>[4x]SMRNVALITGITGQDGSYLAEFLLEKGYEVHGIVRRSSSFNTGRIEHLYKNPQAHIEGNMKLHYGDLTDSTCLVKIINEVKPTEIYNLGAQSHVKISFDLAEYTADVDGVGTLRLLDAVKTCGLINSVKFYQASTSELYGKVQEIPQKETTPFYPRSPYGAAKLYAYWIVVNF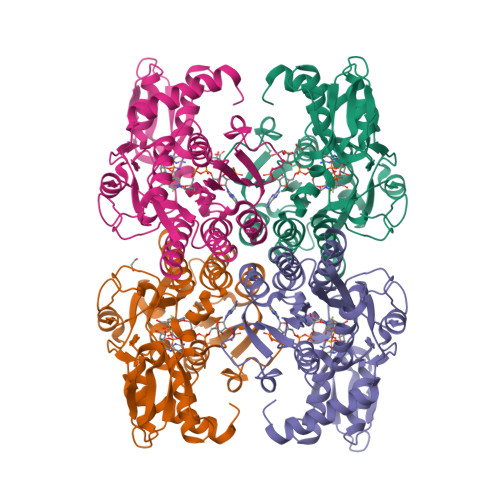REAYNLFAVNGILFNHESPRRGANFVTRKISRSVAKIYLGQLECFSLGNLDAKRDWGHAKDYVEAMWLMLQNDEPEDFVIATGEVHSVREFVEKSFLHIGKTIVWEGKNENEVGRCKETGKVHVTVDLKYYRPTEVDFLQGDCTKAKQKLNWKPRVAFDELVREMVHADVELMRTNPNA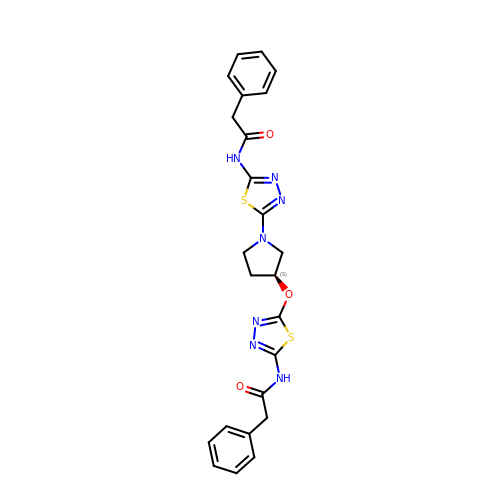2-phenyl-~{N}-[5-[(3~{S})-3-[[5-(2-phenylethanoylamino)-1,3,4-thiadiazol-2-yl]oxy]pyrrolidin-1-yl]-1,3,4-thiadiazol-2-yl]ethanamide | C24 H23 N7 O3 S2 | JGTIIKRXHSZCBG-SFHVURJKSA-N>GCGTAXACGC[2x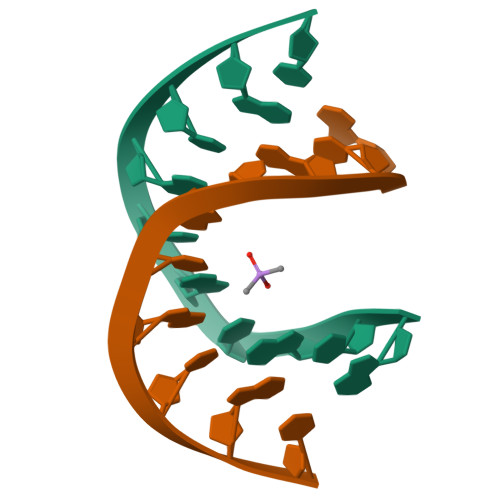]> SHAAILWNEAKAFIAECYAELGKAEEVADRLDSIKSEIDLTGSYVHTKEELEHGAKMAWRNSNRCIGRLFWNSLNVIDRRDVRTKEDVRDALFHHIETATNNGKIRPSITIFPPEEKGEKQVEIWNHQLIRYAGYEGEAIGDPASCSLTAACEQLGWRGERTDFDLLPLIFRMKGDEQPVWYELPRSLVIEVPITHPDIEAFSDLELKWYGVPIISDMKLEVGGIHYNA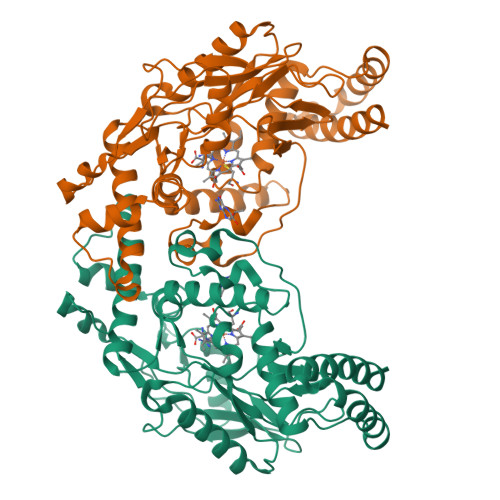APFNGWYMGTEIGARNLADEKRYDKLKKVASVIGISTNYNTDLWKDQALVELNKAVLYSYKKQGVSIVDHHTAASQFKRFEEQEEEAGRKLTGDWTWLIPPISGSATHIFHRSYDNSIVKPNYFYQDKPYE2-chloranyl-6-[(3~{S})-3-[(1~{S})-2-cyano-1-[4-(7~{H}-pyrrolo[2,3-d]pyrimidin-4-yl)pyrazol-1-yl]ethyl]pyrrolidin-1-yl]benzenecarbonitrile | C23 H19 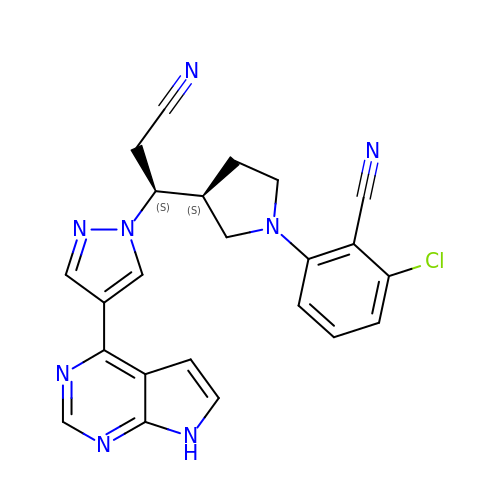Cl N8 | BKUZTJNOISYCFG-YWZLYKJASA-N4-amino-N-(6-methoxypyridin-3-yl)-2-methylquinazoline-8-carboxamide | C16 H15 N5 O2 | 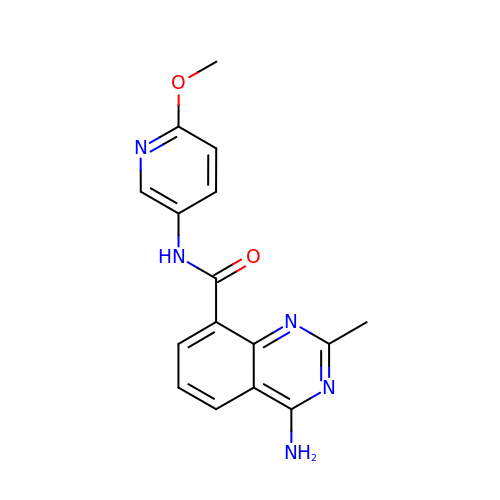IBOOEVQOPIWXHO-UHFFFAOYSA-N> AQIGPVTDLHITNANISPDGFSRPAVLAGGTFPGPTIAGNTGDNFQITVFNDLTDPSMLTDTSIHWHGLFQKGTNWADGPAFVTQCPIITGQSFDYNFNVPGQAGTFWYHSHLSTQYCDGLRGPFVVYDPNDPNASLYDVDDDTTIITLADWYHTLAQQEPIGAAITADATLINGLGRSFTNTTASPLSVITVQSGKRYRMRLVSISCDPNYLFSID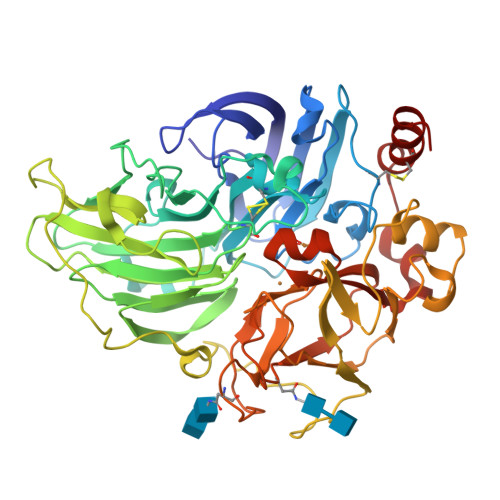GHDMTIIEVDGVNSQQLTVDQIQIFAAQRYSFVLNANQPVGNYWIRAQPNSGGQGFDGGINSAILRYEGATVEDPTTTAPTTFSNPLVETDLHPLADLGVPGQPFRGGADDPLVLNLAFANGRFSIDGVSFVPPTVPVLLQILSGAQNAQDLLPAGSVISLPSNSVIEVALPAGAAGGPHPFHLHGHNFAVVQSANNATPNYVNPIWRDTVSIGGTGDNVTIRFTTNNPGPWFLHCHIDWHLEAGFAIVFAEDIPDTASANPVPQAWSDLCPAYDQAHNISA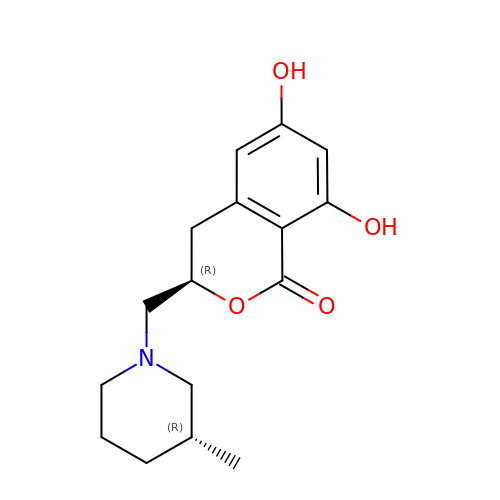(3R)-3-[[(3R)-3-methylpiperidin-1-yl]methyl]-6,8-bis(oxidanyl)-3,4-dihydroisochromen-1-one | C16 H21 N O4 | ZNIKUZOBPQNYBK-ZWNOBZJWSA-N6-(1~{H}-pyrazol-4-yl)pyridine-3-carboxylic acid | C9 H7 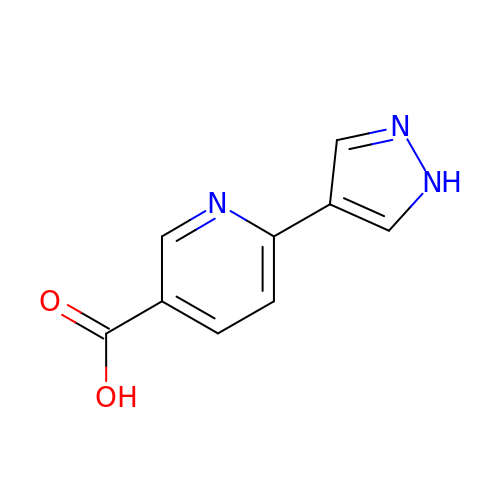N3 O2 | HOWKGKXZKIRBGK-UHFFFAOYSA-N> FPTIPLSRLFDNAMLRAHRLHQLAFDTYQEFEEAYIPKEQKYSFLQNPQTSLCFSESIPTPSNREETQQKSNLELLRISLLLIQSWLEPVQFLRSVFANSLVYGASDSNVYDLLKDLEERIQTLMGRLEDGSPRTGQIFKQTYSKFDTNSHNDDALLKNYGLLYCFRKDMDKVETFLRIVQCRSVEGSCGF;> FSGSEATAAILSRAPWSLQSVNPGLKTNSSKEPKFTKCRSPERETFSCHWTDEVHHGTKNLGPIQLFYTRRNTQEWTQEWKECPDYVSAGENSCYFNSSFTSIWIPYCIKLTSNGGTVDEKCFSVDEIVQPDPPIALNWTLLNVSLTGIH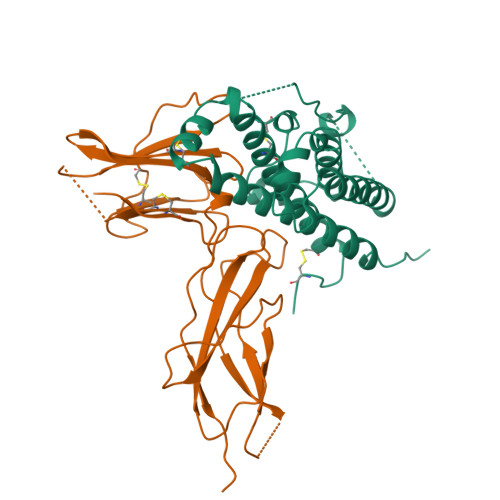ADIQVRWEAPRNADIQKGWMVLEYELQYKEVNETKWKMMDPILTTSVPVYSLKVDKEYEVRVRSKQRNSGNYGEFSEVLYVTLPQMSQ2-methyl-5-(prop-1-en-2-yl)phenol | C10 H12 O | 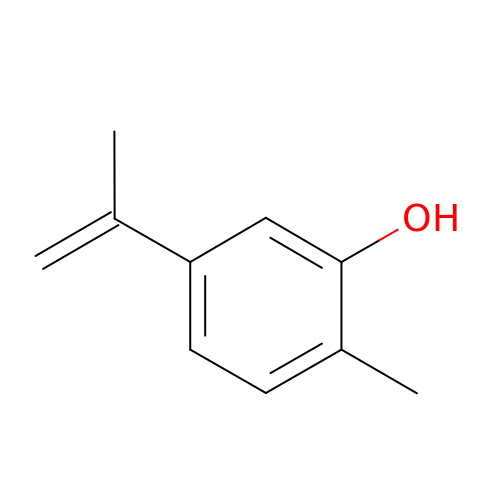HHTWOMMSBMNRKP-UHFFFAOYSA-N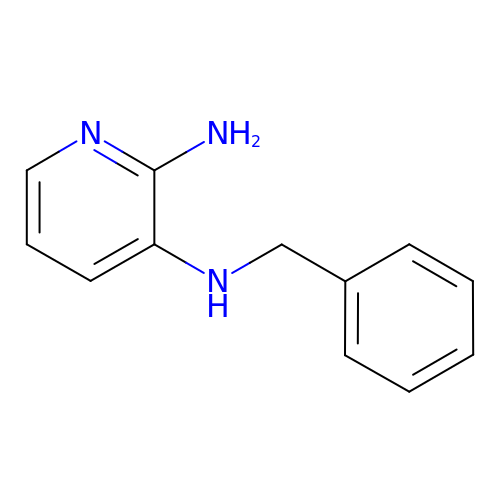N~3~-BENZYLPYRIDINE-2,3-DIAMINE | C12 H13 N3 | MUKAGFLFIMVSQN-UHFFFAOYSA-N>[8x]MTTPYKHEPFTNFGIEENRKAFEKALETVNNEWLGQSYPLVIDGERYETENKIVSINPANKEEVVGTVSKATQDHAEKAIQAAAKAFETWRYTDPEERAAVLFRAVAKVRRKKHEFSALLVKEAGKPWNEADADTAEAIDFMEYYARQMIELAKGKPVNSREGERNQYVYTPTGVTVVIPPWNFLFAIMAGTTVAPIVTGNTVVLKPASAAPVIAAKFVEVLEES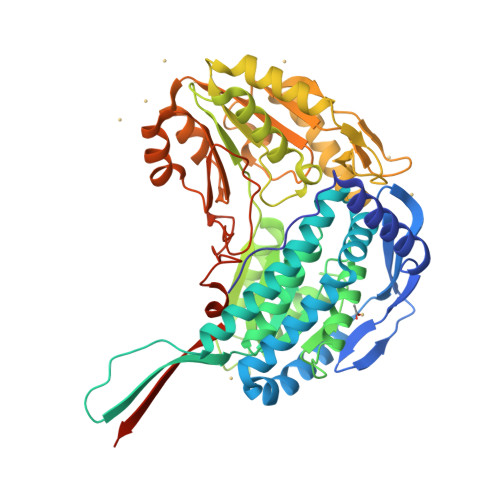GLPKGVVNFVPGSGAEVGDYLVDHPKTSIITFTGSREVGTRIFERAAKVQPGQTHLKQVIAEMGGKDTVVVDEDCDIELAAQSIFTSAFGFAGQKCSAGSRAVVHEKVYDEVLKRVIEITESKKVGEPDSADVYMGPVIDQASFNKIMDYIEIGKEEGRLVSGGKGDDSKGYFIEPTIFADLDPKARLMQEEIFGPVVAFSKVSSFDEALEVANNTEYGLTGAVITKNRDHINRAKQEFHVGNLYFNRNCTGAIVGYHPFGGFKMSGTDSKAGGPDYLALHMQAKTISEMFAENLYFQSHHHHHHWSHPQFEK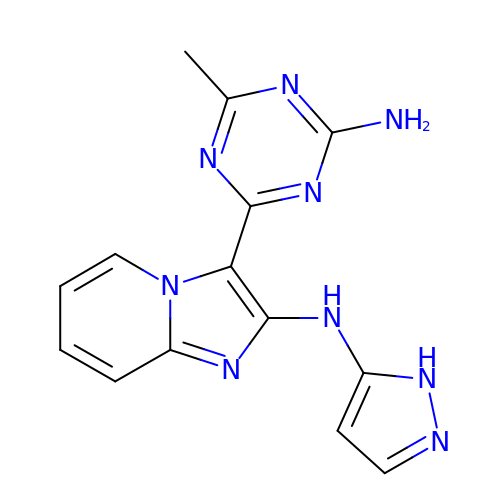3-(4-amino-6-methyl-1,3,5-triazin-2-yl)-N-(1H-pyrazol-5-yl)imidazo[1,2-a]pyridin-2-amine | C14 H13 N9 | OEQWYIZFUDGMEW-UHFFFAOYSA-N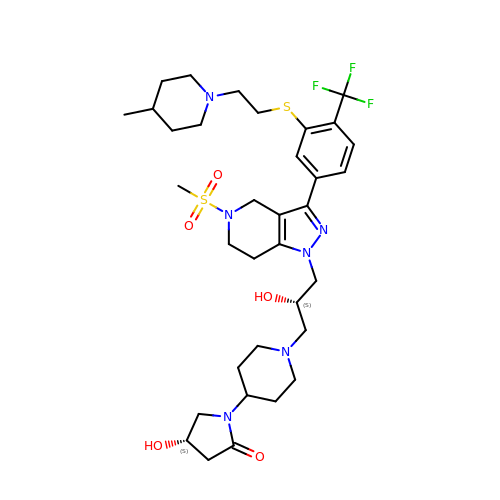(4~{S})-1-[1-[(2~{S})-3-[3-[3-[2-(4-methylpiperidin-1-yl)ethylsulfanyl]-4-(trifluoromethyl)phenyl]-5-methylsulfonyl-6,7-dihydro-4~{H}-pyrazolo[4,3-c]pyridin-1-yl]-2-oxidanyl-propyl]piperidin-4-yl]-4-oxidanyl-pyrrolidin-2-one | C34 H49 F3 N6 O5 S2 | CKJQVJQFVFWPOY-SVBPBHIXSA-N>[4x]SNANCKKIGEDSKIIIRQITDNDLELLMAWRSNPLIYKFFYIQKEPLKWEE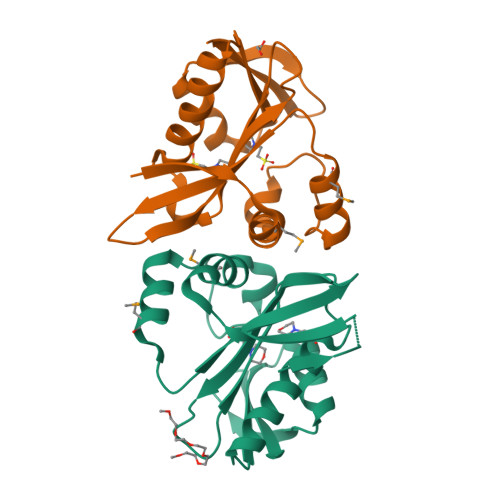HYSWWMSRENRVDWIILLRENNTIRKVGSVNVSQLNTDNPEIGILIGEFFLWGKHIGRHSVSLVLKWLKNIGYKKAHARILENNIRSIKLFESLGFKKTKKGRENEWIYEVNL> MPEESSPRRTPQSIPYQDLPHLVNADGQYLFCRYWAPTGTPKALIFVSHGAGEHSGRYEELARMLMGLDLLVFAHDHVGHGQSEGERMVVSDFHVFVRDVLQHVDSMQKDYPGLPVFLLGHSMGGAIAILTAAERPGHFAGMVLISPLVLANPESATTFKVLAAKVLNSVLPNLSSGPIDSSVLSRNKTEVDIYNSDPLICRAGLKVCFGIQLLNAVSRVERALPKLTVPFLLLQGSADRLCDSKGAYLLMELAKSQDKTLKI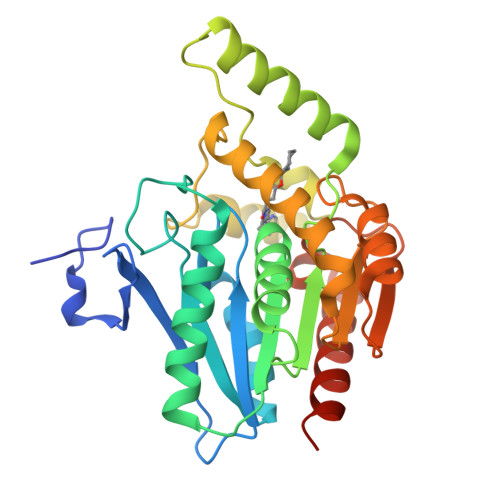YEGAYHVLHKELPEVTNSVFHEINMWVSQRTATAGTASPP> GNSGRFERDAFDTLFDHAPDKLSVVKKSLITFVNKHLNKLNLEVTELETQFADGV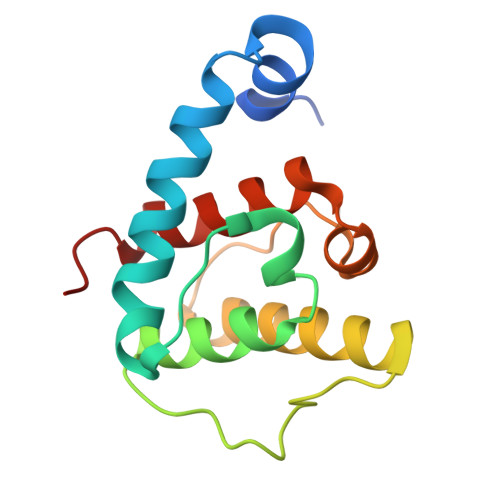YLVLLMGLLEDYFVPLHHFYLTPESFDQKVHNVSFAFELMLDGGLKKPKARPEDVVNLDLKSTLRVLYNLFTKYKNVE>MPVAEQPYHHGSLRRVLLARAESTLEKDGVDGLSLRQLAREAGVSHAAPSKHFRDRQALLDALAESGFLRLTAALERAVEEAESHARARFAALAGAYVSFALAHRELLALMYGNKHAPGAASQVVEAGHASMDLTVRIVTEAQAAGDIGPGDASRIALVAFATFHGIATLAAGGMLDGAPVDEVVT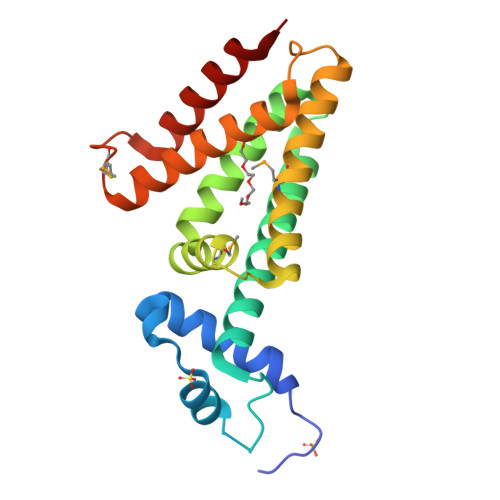AASDTFWRGLAQA[4x]> SGRGK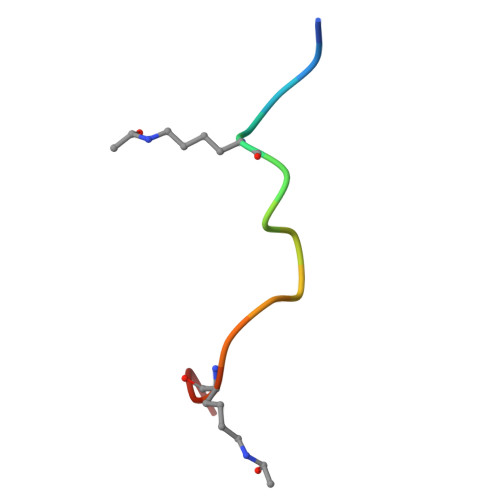GGKGLGKGGA>[2x]MASMTGGQQMGRDQAGITGTWYNQLGSTFIVTAGADGALTGTYESAVGNAESRYVLTGRYDSAPATDGSGTALGWTVAWKNNYRNAHSATTWSGQYVGGA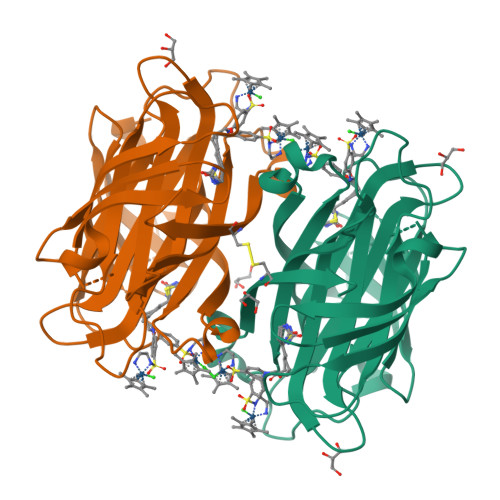EARINTQWLLTSGTTEANAWASTLVGHDTFTKVKPSAASIDAAKKAGVNNGNPLDAVQQGSGGGNGGGNGGGNGGGNIDGRGGGNASMTGGQQMGRDQAGITGTWYNQLGSTFIVTAGADGALTGTYVTARGNAESRYVLTGRYDSAPATDGSGTALGWTVAWKNNYRNAHSATTWSGQYVGGAEARINTQWLLTSGTTEANAWKSTLVGCDTFTKVKPSAASIDAAKKAGVNNGNPLDAVQQ Here, we discover a family of Bdellovibrio proteins that define a new subgrouping of the lysozyme superfamily and demonstrate that they possess outright specificity for deacetylated peptidoglycan. We solve the structure of family member Bd0314 (that we named DslA), revealing adaptations to the lysozyme fold that sterically restrict the active-site cleft into only accepting polymers deacetylated at the GlcNAc positions. We determine a role for DslA in B. bacteriovorus exit from the prey cell and demonstrate that exogenously added enzyme is able to prematurely liberate predators from prey bdelloplasts before completion of the predatory lifecycle. The architecture of DslA is related to, but significantly different from, other members of the lysozyme superfamily but still fulfil the inclusion criteria for the lysozyme superfamily noted by Monzingo et al. — conservation of the β-sheet floor and helices D and F, with appropriate placement of acidic catalytic residues.

We were able to successfully purify the enzymatic domain of DslA by omitting the lipobox and ~35 aa region of low complexity/disorder, fusing region R74-K254 to maltose-binding protein (later cleaved). This construct yielded two independent crystal forms, diffracting to 1.26 and 1.36 Å resolution. Attempts to solve these via molecular replacement with “conventional” lysozyme structures failed, indicating potential divergence from the superfamily fold.Table. All four of our DslA structures (two wild-type, E143Q, E154Q) are highly similar, other than a relatively small flexation of the β1–2 hairpin in the E154Q variant. The secondary structure elements create a classical two-lobed architecture, with helix E and β1–2 sat below a pronounced active-site cleft (measuring ~25 Å across, ~15 Å deep). Partial activity for HEWL against the GlcNAc-deacetylase-treated material was indicative of our in vitro prior deacetylation of E. coli PG not running to completion, and illustrative of the difficulties of reconstituting B. bacteriovorus activities in vitro outside of the bdelloplast. Despite this, DslA was clearly inactive against native, acetylated peptidoglycan, but displayed strong activity against the deacetylated material; this level of activity was on a similar scale to that of HEWL and mutanolysin with their known substrates. Of the six saccharide rings, GlcNAc “c” and “e” sit with the 2′-NAc groups facing inward. These two positions are occupied in DslA by Y228 and M150, the former placing the sidechain OH in the same position as an acetyl oxygen. Hence, specificity of DslA for GlcN over GlcNAc presumably arises via steric blockage of ring c and e if the sugar groups are acetylated.

> MKNTPQHKLFFVVALLLVVQILAGCKSSSSTTAGSTENSSSSTPDPDTGTTTPDPIEPEVVPPVTPPSVDSNSREVIPLWEDKVADGKAWSTHVYSALDKLGPNLLDVIPADRSLFCPKYSSLSYAQRKQYWAFVLSSMVRFESNFKTAMSYTEDFNDSNGNRVISRGLLQISIESGNAYGCGFKSTKDLHDPLQNLSCGIRILDRWVSRDGRIAGKVDGAWKGGARYWSVLRAGDKTSYKSIVSWSQNLSICK1-butylisochromeno[3,4-c]pyrazol-5(3H)-one | C14 H14 N2 O2 | 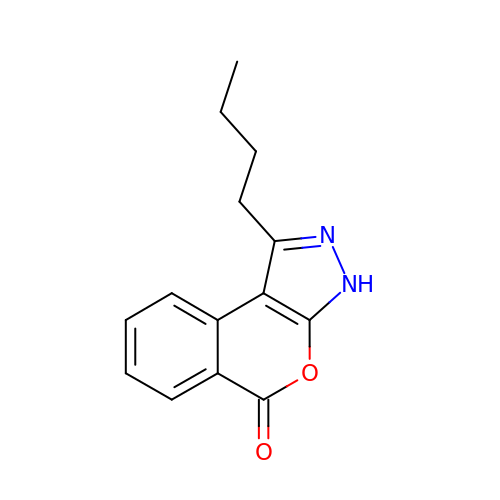YKYPXFBQABKRKC-UHFFFAOYSA-N>[18x]XSKLL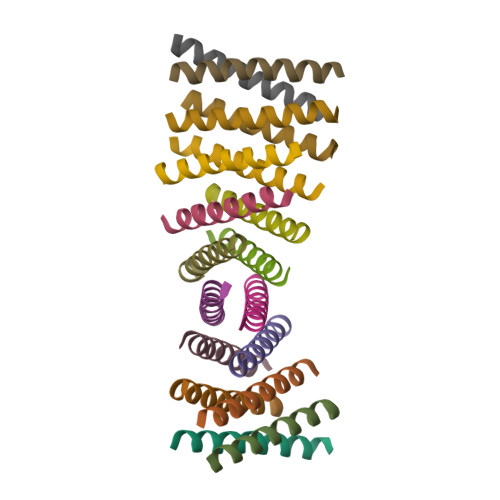ELLRKLGEALHKAIELLEKWGX> DES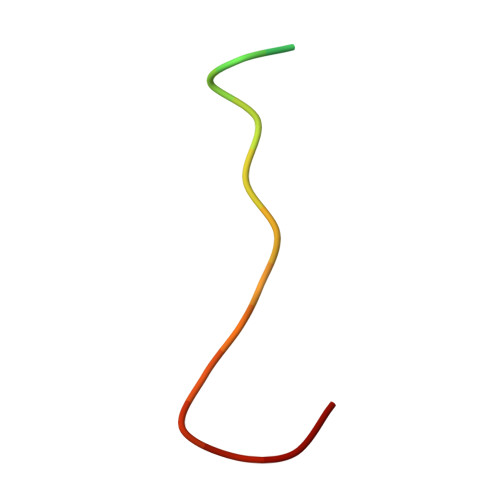GLPQLTSYDAEVNAPI> GPGAPNVLNWEQVQRLDG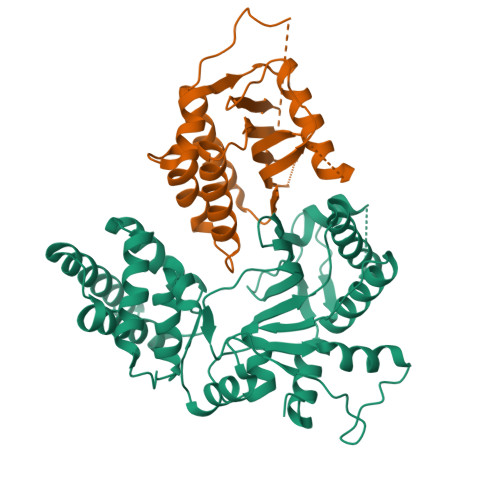ILSETIPIHGRGNFPTLELQPSLIVKVVRRRLAEKRIGVRDVRLNGSAASHVLHQDSGLGYKDLDLIFCADLRGEGEFQTVKDVVLDCLLDFLPEGVNKEKITPLTLKEAYVQKMVKVCNDSDRWSLISLSNNSGKNVELKFVDSLRRQFEFSVDSFQIKLDSLLLFYECSENPMTETFHPTIIGESVYGDFQEAFDHLCNKIIATRNPEEIRGGGLLKYCNLLVRGFRPASDEIKTLQRYMCSRFFIDFSDIGEQQRKLESYLQNHFVGLEDRKYEYLMTLHGVVNESTVCLMGHERRQTLNLITMLAIRVLADQNV;> GPGAPDEVIDEEVNIEFEAYSLSDNDYDGIKKLLQQLFLKAPVNTAELTDLLIQQNHIGSVIKQTDVSEDSNDDMDEDEVFGFISLLNLTERKGTQCVEQIQELVLRFCEKNCEKSMVEQLDKFLNDTTKPVGLLLSERFINVPPQIALPMYQQLQKELAGAHRTNKPCGKCYFYLLISKTFVEAGKNNSKKKPSNKKKAALMFANAEEEFFYEEQGKPEVLGGPDTRRGLEPVPIQHNGGSRGQVTALVSLKAGLIQSRSTLSDFQGTFMTVGIALS>MMEQVCDVFDIYAICVCCKVESKNEGKKNEVFNNYTFRGLGNKGVLPWKCNSLDMKYFCAVTTYVNESKYEKLKYKRCKYLNKETVDNVNDMPNSKKLQNVVVMGRTTWESIPKKFKPLSNRINVILSRTLKKEDFDEDVYIINKVEDLIVLLGKLNYYKCFIIGGSVVYQEFLEKKLIKKIYFTRINSTYECDVFFPEINENEYQIISVSDVYTSNNTTLDFIIYKKTNNKMLNEQNCIKGEEKNNDMPLKNDDKDTCHMKKLTEFYKNVDKYKINYENDDDDEEEDDFVYFNFNKEKEEKNKNSIHPNDFQIYNSLKYKYHPEYQYLNIIYDIMMNGNKQSDRTGVGVLSKFGYIMKFDLSQYFPLLTTKKLFLRGIIEELLWFIRGETNGNTLLNKNVRIWEANGTREFLDNRKLFHREVNDLGPIYGFQWRHFGAEYTNMYDNYENKGVDQLKNIINLIKNDPTSRRILLCAWNVKDLDQMALPPCHILCQFYVFDGKLSCIMYQRSCDLGLGVPFNIASYSIFTHMIAQVCNLQPAQF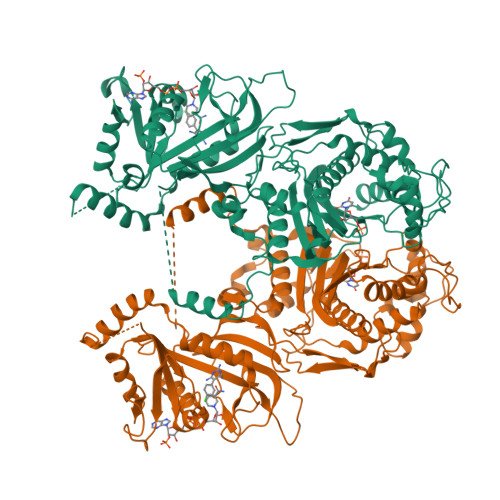IHVLGNAHVYNNHIDSLKIQLNRIPYPFPTLKLNPDIKNIEDFTISDFTIQNYVHHEKISMDMAA[2x]>VESLMQALPGIGWTAALLLMMFYIFAVMGTELFGEAFPQWFGSLGASIYSLFQIMTLESWSMGIARPVMEVYPLAWIFFVPFILISSFMVLNLFIAIIVSATQEVHESEQRAEREANNLIAHDERQEMLDLMRAMHAKI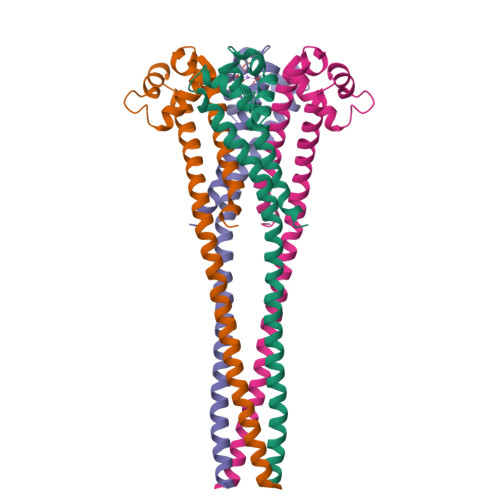VALEQQGKAGQ[8x]Chronic myeloid leukemia (CML) is the result of the constitutive kinase activity of the tyrosine kinase BCR-Abl, the product of the bcr-abl gene fusion present on the Philadelphia chromosomes of patients with CML. Bosutinib is a second-generation dual Abl/Src inhibitor that exhibits potent growth inhibition of CML cells in vitro, is active against multiple imatinib-resistant BCR-Abl mutations and has demonstrated efficacy in ongoing clinical trials for imatinib-resistant CML. In the course of studies of electrostatic interactions in the ATP-binding sites of several kinases, briefly outlined at the end of this report, we determined the crystal structure of the kinase domain of Abl bound to bosutinib at 2.4 angstrom resolution. The structure explains the effects of imatinib resistance mutations on bosutinib binding, and provides a basis for interpreting spectroscopic measurements that probe the environment of the ATP-binding site of Abl and other kinases.

Crystals of Abl kinase domain bound to the compound from Tocris Bioscience were obtained in the same crystal form, and we solved the structure to a resolution of 2.4 angstroms. Anomalous difference maps calculated using the phases from the refined molecular model show strong peaks (greater than 4 standard deviations above the mean) for the chlorine atoms of the drug in the ortho and para positions on the aniline ring, confirming the identity of the compound. Bosutinib occupies the ATP-binding site of Abl, sandwiched between the N-terminal and C-terminal lobes of the kinase. The only hydrogen bond formed between bosutinib and Abl is between the quinoline N1 nitrogen atom and the backbone amide of M318 (a residue in the hinge region of the kinase), a characteristic feature of the binding mode of this class of inhibitors. The 2,4-dichloro-5-methoxy aniline fragment of bosutinib is oriented at a ∼65° angle to the plane of the quinoline heterocycle and fills a hydrophobic pocket formed by residues projecting from the N-lobe into the ATP-binding site. The sidechain of T315 is completely enveloped by bosutinib, making extensive van der Waals contacts with both the nitrile group and the 5-methoxy group of the aniline ring. The nitrile group is also in van der Waals contact with the sidechain of V299. Both the T315I and V299L mutations would result in steric clashes with bosutinib, explaining why these mutations confer resistance to bosutinib. In our structure of Abl bound to bosutinib two residues at the tip of the P-loop (Q252 and Y253) are poorly ordered, but the remainder of the loop adopts an extended conformation similar to the β-hairpin observed in a substrate complex of Abl and makes no contacts with bosutinib. In our structure of Abl bound to bosutinib, the DFG motif is in an inactive DFG-Out conformation, but this conformation is distinct from the DFG-Out conformation observed in complex with imatinib.

>[2x]GHMSPNYDKWEMERTDITMKHKLGGGQYGEVYEGVWKKYSLTVAVKTLKEDTMEVEEFLKEAAVMKEIKHPNLVQLLGVCTREPPFYIITEFMTYGNLLDYLRECNRQEVNAVVLLYMATQISSAMEYLEKKNFIHRDLAARNCLVGENHLVKVADFGLSRLMTGDTYTAHAGAKFPIKWTAPESLAYNKFSIKSDVWAFGVLLWEIATYGMSPYPGIDLSQVYELLEKDYRMERPEGCPEKVYELMRACWQWNPSDRPSFAEIHQAFETMFQESSISDEVEKELGK> MSEPRFVHLRVHSDYSMIDGLAKTAPLVKKAAALGMPALAITDFTNLCGLVKFYGAGHGAGIKPIVGADFNVQCDLLGDELTHLTVLAANNTGYQNLTLLISKAYQRGYGAAGPIIDRDWLIELNEGLILLSGGRMGDVGRSLLRGNSALVDECVAFYEEHFPDRYFLELIRTGRPDEESYLHAAVELAEARGLPVVATNDVRFIDSSDFDAHEIRVAIHDGFTLDDPKRPRNYSPQQYMRSEEEMCELFADIPEALANTVEIAKRCNVTVRLGEYFLPQFPTGDMSTEDY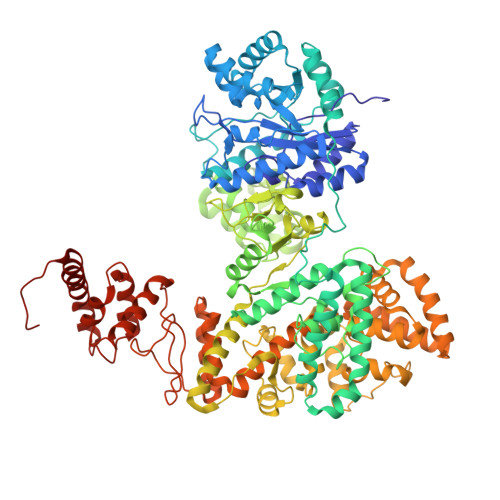LVKRAKEGLEERLAFLFPDEEERLKRRPEYDERLETELQVINQMGFPGYFLIVMEFIQWSKDNGVPVGPGRGSGAGSLVAYALKITDLDPLEFDLLFERFLNPERVSMPDFDVDFCMEKRDQVIEHVADMYGRDAVSQIITFGTMAAKAVIRDVGRVLGHPYGFVDRISKLIPPDPGMTLAKAFEAEPQLPEIYEADEEVKALIDMARKLEGVTRNAGKHAGGVVIAPTKITDFAPLYCDEEGKHPVTQFDKSDVEYAGLVKFDFLGLRTLTIINWALEMINKRRAKNGEPPLDIAAIPLDDKKSFDMLQRSETTAVFQLESRGMKDLIKRLQPDCFEDMIALVALFRPGPLQSGMVDNFIDRKHGREEISYPDVQWQHESLKPVLEPTYGIILYQEQVMQIAQVLSGYTLGGADMLRRAMGKKKPEEMAKQRSVFAEGAEKNGINAELAMKIFDLVEKFAGYGFNKSHSAAYALVSYQTLWLKAHYPAEFMAAVMTADMDNTEKVVGLVDECWRMGLKILPPDINSGLYHFHVNDDGEIVYGIGAIKGVGEGPIEAIIEARNKGGYFRELFDLCARTDTKKLNRRVLEKLIMSGAFDRLGPHRAALMNSLGDALKAADQHAKAEAIGQLDLFGVL>GPAVRTIRIYQPGEYQPGQLLELSPEAGQHVGVVLRMEQGEQLTLFNGDNKEFTASIERVKKKQVFVRIASVLEVNRESPLKIHLAQAISKGERMEMVMQKSAELGVACITPLITERCQVKIDKEKMAKKMHQWLNIIIG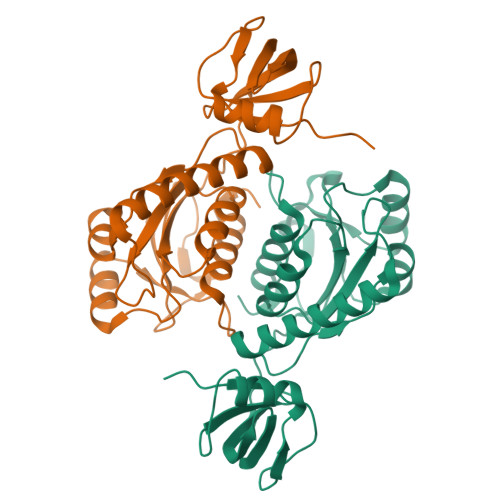ACEQCGRNQIPELRQPVYLDQFVREAKEHLKLILHPAFSKTWRDYPVQPPDVALIIGPEGGFSDEEIRLTSGHGFLPLSLGPRVLRTETAAITALSVLQAAGGDL[4x]> MSFINYSSREINCKIVYYGPGLCGKTTNLQYIYNKTAAETKGKLISLSTETDRTLFFDFLPLSLGEIRGFKTRFHLYTVPGQVFYDASRKLILKGVDGVVFVADSQIERMEANMESLENLRINLAEQGYDLNKIPYVIQYNKRDLPNAVTVEEMRKALNHRNIPEYQAVAPTGVGVFDTLKAVAKLVLTELKKGGHHHH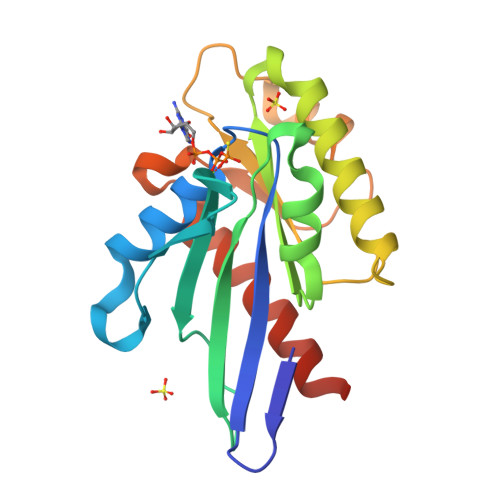HH>[4x]GQMQQASTPTIGMIVPPAAGLVPADGARLYPDLPFIASG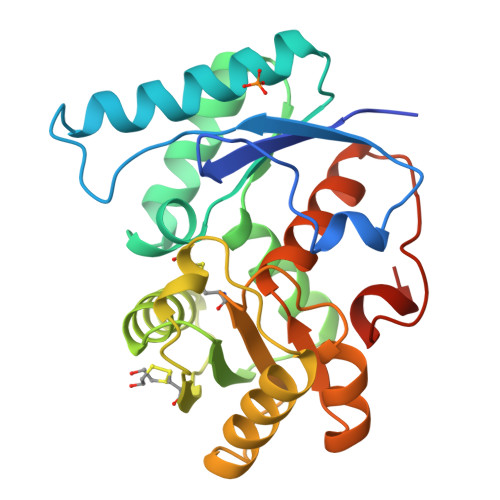LGLGSVTPEGYDAVIESVVDHARRLQKQGAAVVSLMGTSLSFYRGAAFNAALTVAMREATGLPCTTMSTAVLNGLRALGVRRVALATAYIDDVNERLAAFLAEESLVPTGCRSLGITGVEAMARVDTATLVDLCVRAFEAAPDSDGILLSCGGLLTLDAIPEVERRLGVPVVSSSPAGFWDAVRLAGGGAKARPGYGRLFDESGGSHHHHHH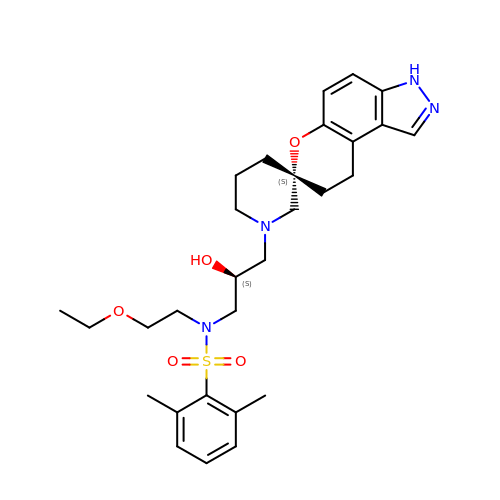N-{(2S)-3-[(3S)-8',9'-dihydro-1H,3'H-spiro[piperidine-3,7'-pyrano[3,2-e]indazol]-1-yl]-2-hydroxypropyl}-N-(2-ethoxyethyl)-2,6-dimethylbenzenesulfonamide | C29 H40 N4 O5 S | ZSKFBGIRLVOQAD-MUAVYFROSA-N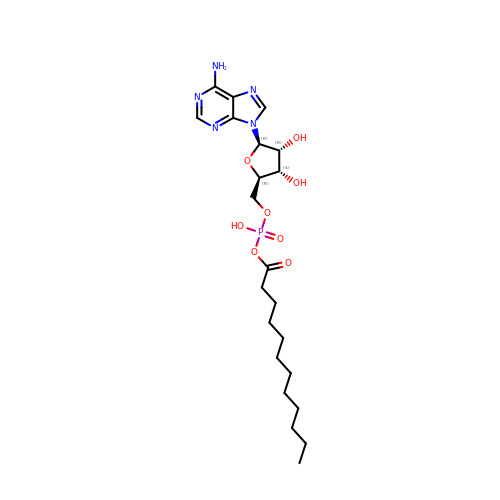5'-O-[(S)-(dodecanoyloxy)(hydroxy)phosphoryl]adenosine | C22 H36 N5 O8 P | IKBWVSPLSBIYSK-CIVUBGFFSA-N> MAIVRVHYKIYGRVQGVGFRWSTQREGRKLGLNGWVRNL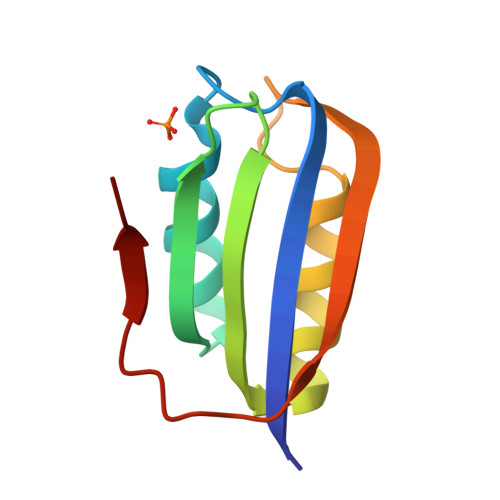PDGSVEGVLEGDEERVEAMIGWLHQGPPLARVTRVEVKWEQPKGEKGFRIVG> MGYYDEDGHYHSFRQGIHKLADKIAHPHHHHHDHVDVDIKEDIRVTETRPRPVQSGGSYVPNTVTIPCHHIRLGDFLMLQGRPCQVIRISTSNATGQYRYLGVDLFTKQLHEESSFV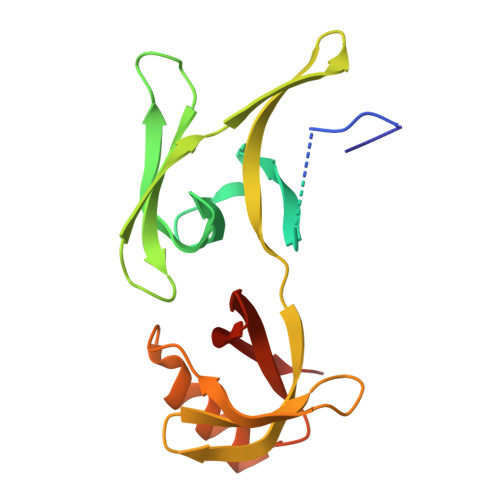SNPAPSVIVQTMLGPVFKQYRVLDMQGGHIVAMTETGDVKQSLPVIDQSNLWSRLSTAFESGRGSVRVLVLNDSGRELAVDMKVIHGSRL> EQPEPIKVYGQVSLNDSHNQMVVHWAGEKSNVIVALARDSLALARPKSSDVYVSYDYGKSFKKISDKLNFGLGNRSEAVIAQFYHSPADNKRYIFADAYAQYLWITFDFCNTLQGFSIPFRAADLLLHSKASNLLLGFDRSHPNKQLWKSDDFGQTWIMIQEHVKSFSWGIDPYDKPNTIYIERHEPSGYSTVFRSTDFFQSRENQEVILEEVRDFQLRDKYMFATKVVHLLGSEQQSSVQLWVSFGRKPMRAAQFVTRHPINEYYIADASEDQVFVCVSHSNNRTNLYISEAEGLKFSLSLENVLYYSPGGAGSDTLVRYFANEPFADFHRVEGLQGVYIATLINGSMNEENMRSVITFDKGGTWEFLQAPAFTGYGEKINCELSQGCSLHLAQRLSQLLNLQLRRMPILSKESAPGLIIATGSVGKNLASKTNVYISSSAGARWREALPGPHYYTWGDHGGIITAIAQGMETNELKYSTNEGETWKTFIFS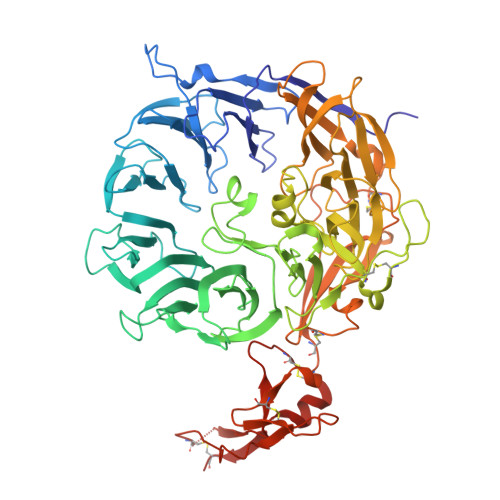EKPVFVYGLLTEPGEKSTVFTIFGSNKENVHSWLILQVNATDALGVPCTENDYKLWSPSDERGNECLLGHKTVFKRRTPHATCFNGEDFDRPVVVSNCSCTREDYECDFGFKMSEDLSLEVCVPDPEFSGKSYSPPVPCPVGSTYRRTRGYRKISGDTCSGGDVEARLEGELVPCPSRLENLYFQ Virulent phages belonging to the newly created Skunavirus genus (previously 936) are by far the most predominant in dairy factories and they currently belong to the Siphoviridae family (double-stranded DNA genome and non-contractile tail) of the Caudovirales order. Phage p2 is the model phage for this viral genus and it infects L. lactis MG1363, a laboratory strain used in many studies on Gram-positive bacteria. Of interest here, phage p2 uses a multi-protein baseplate at the tip of its tail to bind to its cell wall polysaccharide (CWPS) receptor at the host cell surface. Here, we present further structural analyzes of the phage p2 baseplate, proposing a topological model of the baseplate resting state, and interpreting a new nsEM structure of the virion, in its active conformation.

Thus, we were able to build an atomic model of the baseplate containing the distal tail protein (Dit, ORF15), the tail associated lysin protein (Tal, ORF16), and the RBP complexed by VHH5 binders. We also determined the cryo-electron microscopy (cryoEM) structure of a freshly purified and glutaraldehyde cross-linked baseplate at 26 Å resolution. The baseplate architectures in the cross-linked complex and in the native p2 virions were similar within their resolution limit. Furthermore, the overall architecture of the baseplate crystal structure, depleted of the VHH5s, was in agreement with the EM structures. However, the baseplate atomic model containing six Dit, three Tal and six trimers of RBP corresponded only to a part of the cross-linked baseplate EM structure, as a two ring-shaped density could not be immediately assigned to any component of the structure. Since the recombinantly produced baseplate contained only Dit, Tal, and RBP, these densities had to be fulfilled by one of the three components, and a second Dit hexamer was the most likely candidate. Therefore, we proposed that one of the rings could be formed by a Dit N-terminal domain back to back with the first Dit N-terminal domain (referred to as Dit-1) hexameric ring, while the second ring (referred to as Dit-2) could be formed by the Dit C-terminal galectin domains, rearranged to form a hexamer. We noticed that small densities point out of Dit-2 galectin ring and contact the RBPs, probably keeping the baseplate in a resting state. In the baseplate crystal structure, the RBP orientation was somewhat surprising since the receptor-binding domains were found to point towards the virion capsid and not in the opposite direction, as intuitively thought to interact with the host cell wall receptor. In both baseplate conformations, an extension of the Dit galectin domain, the “arm”, holds the RBPs by inserting its “hand” within the trimeric RBP “shoulder” domain.

>[3x]MLEANVYDNFNPNYYNISDFSMPNGKKEKRGLPIPKARCQVINYELWETGYLYTSSATLTVSVEVGDIVQILFPEVVPIEEALGKKKKLNLDMVYLVTDVDESNKATLKNYFWAMIESLDVPNAITKTTNFAIIDYLIDPNKNNLMSYGYFFNSSIFAGKATINRKAETSSAHDVAKRIFSKVQFQPTTTIQHAPSETDPRNLLFINFASRNWNRKRITTRVDIKQSVTMDTETIVERSAYNFAVVFVKNKATDDYTDPPKMYIAKNNGDVIDYSTYHGDGTDLPDVRTAKTLFYDRDDHGNPPELSTIKVEISPSTIVTRLIFNQNELLPLYVNDLVDIWYEGKLYSGYIADRVKTEFNDRLIFVESGDKPNVI;>[12x]MVRQYKIHTNLDGTDDKVWDVTNGKVRFYQPSNLGLQSTNNIWQSNGIGVMGTRSITQPQIEFKLETFGESLEENYQLMKDFVNDILSKKFVTLEYQTEIFQVYADLALADVTKTEGYGKNGTFSEKITFDIITKWYTYENLTFDKIQNGKVIAGMSKIYGGTAPGNYKYIKGTSYTYYGESDIDRLSRWDIKEEIFSFMGILYPKLPKTPAGVRFLDDIGNEYTAIVFKTEQVQDYILINTDVNDETYQGWKGTTALNLFPVMDFERYRTRIIEKGQMELINLSKAEFKIKRKADFV;>[18x]MTIKNFTFFSPNSTEFPVGSNNDGKLYMMLTGMDYRTIRRKDWSSPLNTALNVQYTNTSIIAGGRYFELLNETVALKGDSVNYIHANIDLTQTANPVSLSAETANNSNGVDINNGSGVLKVCFDIVTTSGTGVTSTKPIVQTSTLDSISVNDMTVSGSIDVPVQTLTVEAGNGLQLQLTKKNNDLVIVRFFGSVSNIQKGWNMSGTWVDRPFRPAAVQSLVGHFAGRDTSFHIDINPNGSITWWGANIDKTPIATRGNGSYFIK> MSTLAQQALHNNNVGPIIRAGDLVEPVIETAEIDNPGKEIT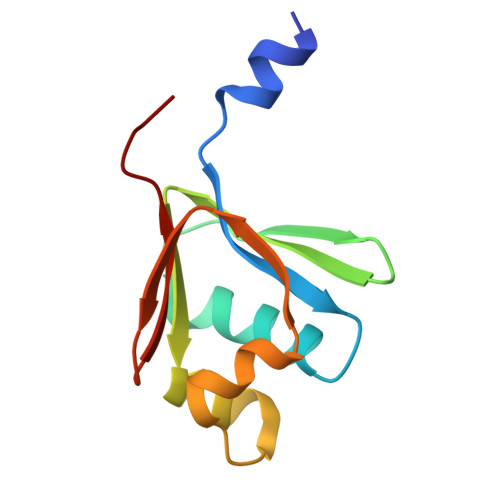VEDRRAYVRIAAEGELILTRKTLEEQLGRPFNMQELEINLASFAGQIQADEDQIRFYFDKTM>GAHMFKIPGFGKAAANHTPPDMTNMDTRTRHLKVSNCPNNSYALANVAAVSPNDFPNNIYIIIDNLFVFTTRHSNDIPPGTIGFNGNQRTWGGWSLNQDVQAKAFDLFKYSGKQSYLGSIDIDISFRARGKAVSTVFDQDELAKQFVRCYESQIFSPTQYLIMEFQGHFFDLKIRNVQAIDLGDIEPTSAVATGIETKGILTKQTQINFFKGRDGLVNLKSSNSLRPRSNAVIRPDFKFEDLGVGGLDKEFTKIFRRAFASRIFPPSVIEKLGISHVKGLLLYGPPGTGKTLIARKIGTMLNAKEPKIVNGPEILSKYVGSSEENIRNLFKDAEAEYRAKGEESSLHIIIFDELDSVFKQRGSRGDGTGVGDNVVNQLLAKMDGVDQLNNILVIGMTNRKDLIDSALLRPGRFEVQVEIHLPDEKGRLQIFDIQTKKMRENNMMSDDVNLAELAALTKNFSGAEIEGLVKSASSFAINKTVNIGKGATKLNTKDIAKLKVTREDFLNALNDVTPAFGISEEDLKTCVEGGMMLYSERVNSILKNGARYVRQVRESDKSRLVSLLIHGPAGSGKTALAAEIALKSGFPFIRLISPNELSGMSESAKIAYIDNTFRDAYKSPLNILVIDSLETLVDWVPIGPRFSNNILQMLKVALKRKPPQDRRLLIMTTTSAYSVLQQMDILSCFDNEIAVPNMTNLDELNNVMIESNFLDDAGRVKVINELSRSCPNFNVGIKKTLTNIETARHDEDPVNELVELMTQSA[7x]

SNARE (soluble N-ethylmaleimide-sensitive factor (NSF) attachment protein receptor) proteins drive membrane fusion at different cell compartments as their core domains zipper into a parallel four-helix bundle. After fusion, these bundles are disassembled by the AAA+ (ATPase associated with diverse cellular activities) protein Sec18/NSF and its adaptor Sec17/α-SNAP to make them available for subsequent rounds of membrane fusion. The disassembly requires multiple ATP hydrolysis events in the presence of Mg2+; as few as six ATP hydrolysis events are sufficient. The side-loading and side-release mechanism explains how Sec18/NSF can disassemble SNAREs with constrained topologies.

To address this topological challenge, we next determined structures of the y20S complex after initiating Sec18 hydrolysis by adding Mg2+ (referred to as the ‘hydrolyzing condition’). Informed by a fluorescent protein disassembly assay, we initiated the disassembly reaction and waited 7 s before sample vitrification. The D1 ring is also flat in all these substrate-free classes, with all D1 protomers bound to ADP. This uniform binding to ADP, as opposed to the spiral staircase of apo, ADP-bound and ATP-bound protomers, likely explains the flattened nature of the protomers. In the D2 ring, all protomers are still ATP bound, consistent with their role in oligomerization. Class 4 consists of a configuration where both D1 and D2 rings are heptameric and class 3 is similar to this heptameric class, except that the seventh protomer is only partially occupied. We observed heptameric states of Sec18 and NSF, split-open hexameric states of Sec18 and NSF and a transition between split hexamer and heptamer of Sec18. Hydrolysis likely accelerates the transition from hexameric to heptameric state through the split-open state for two related reasons. First, while ring splitting itself is hydrolysis independent, hydrolysis is associated with large-scale conformational change in the ATPase rings and likely increases the frequency of sampling the open state.> GSHMKRNYILGLDIGITSVGYGIIDYETRDVIDAGVRLFKEANVENNEGRRSKRGARRLKRRRRHRIQRVKKLLFDYNLLTDHSELSGINPYEARVKGLSQKLSEEEFSAALLHLAKRRGVHNVNEVEEDTGNELSTKEQISRNSKALEEKYVAELQLERLKKDGEVRGSINRFKTSDYVKEAKQLLKVQKAYHQLDQSFIDTYIDLLETRRTYYEGPGEGSPFGWKDIKEWYEMLMGHCTYFPEELRSVKYAYNADLYNALNDLNNLVITRDENEKLEYYEKFQIIENVFKQKKKPTLKQIAKEILVNEEDIKGYRVTSTGKPEFTNLKVYHDIKDITARKEIIENAELLDQIAKILTIYQSSE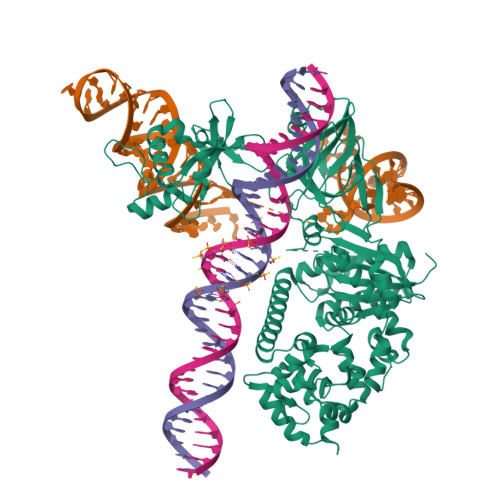DIQEELTNLNSELTQEEIEQISNLKGYTGTHNLSLKAINLILDELWHTNDAQIAIFNALKLVPKKVDLSQQKEIPTTLVDDFILSPVVKRSFIQSIKVINAIIKKYGLPNDIIIELAREKNSKDAQKMINEMQKRNRQTNERIEEIIRTTGKENAKYLIEKIKLHDMQEGKCLYSLEAIPLEDLLNNPFNYEVDHIIPRSVSFDNSFNNKVLVKQEENSKKGNRTPFQYLSSSDSKISYETFKKHILNLAKGKGRISKTKKEYLLEERDINRFSVQKDFINRNLVDTRYATRGLMNLLRSYFRVNNLDVKVKSINGGFTSFLRRKWKFKKERNKGYKHHAEDALIIANADFIFKEWKKLDKAKKVMENQMFEEKQAESMPEIETEQEYKEIFITPHQIKHIKDFKDYKYSHRVDKKPNRKLINDTLYSTRKDDKGNTRIVNNLNGLYDKDNDKLKKLINKSPEKLLMYHHDPQTYQKLKLIMEQYGDEKNPLYKYYEETGNYLTKYSKKDNGPVIKKIKYYGNKLNAHLDITDDYPNSRNKVVKLSLKPYRFDVYLDNGVYKFVKVNNLDVIKKENYYEVNSKCYEEAKKLKKISNQAEFIASFYRNDLIKINGELYRVIGVASDLLNAIEVNMIDITYREYLENMNDKRPPRIFKTISSKTQSIKKYSTDILGNLYEVKSKKHPQIIKKG> GKAFDDGAFTGIREINLSYNKETAIGDFQVVYDLNGSPYVGQNHVSFITG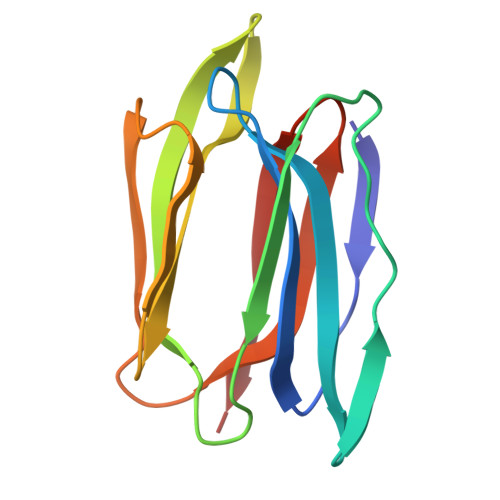FTPVKISLDFPSEYIMEVSGYTGNVSGYVVVRSLTFKTNKKTYGPYGVTSGTPFNLPIENGLIVGFKGSIGYWLDYFSMYLSL> MKFAEHLSAHITPEWRKQYIQYEAFKDMLYSAQDQAPSVEVTDEDTVKRYFAKFEEKFFQTCEKELAKINTFYSEKLAEAQRRFATLQNELQSSLDAQKESTGVTTLRQRRKPVFHLSHEERVQHRNIKDLKLAFSEFYLSLILLQNYQNLNFTGFRKILKKHDKILETSRGADWRVAHVEVAPFYTCKKINQLISETEAVVTNELEDGDRQKAMKRLRVPPLGAAQPAPAWTTFRVGLFCGIFIVLNITLVLAAVFKLETDRSIWPLIRIYRGGFLLIEFLFLLGINTYGWRQAGVNHVLIFELNPRSNLSHQHLFEIAGFLGILWCLSLLACFFAPISVIPTYVYPLALYGFMVFFLINPTKTFYYKSRFWLLKLLFRVFTAPFHKVGFADFWLADQLNSLSVILMDLEYMICFYSLELKWDESKGLLPNNSEESGICHKYTYGVRAIVQCIPAWLRFIQCLRRYRDT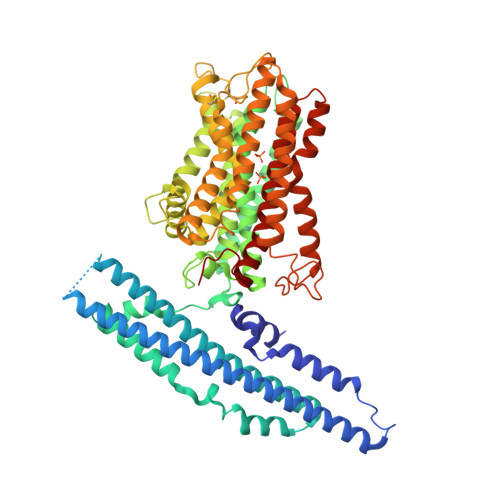KRAFPHLVNAGKYSTTFFMVTFAALYSTHKERGHSDTMVFFYLWIVFYIISSCYTLIWDLKMDWGLFDKNAGENTFLREEIVYPQKAYYYCAIIEDVILRFAWTIQISITSTTLLPHSGDIIATVFAPLEVFRRFVWNFFRLENEHLNNCGEFRA~{N}-[[2,4-bis(fluoranyl)phenyl]methyl]-4-[(4-methylpiperazin-1-yl)methyl]aniline 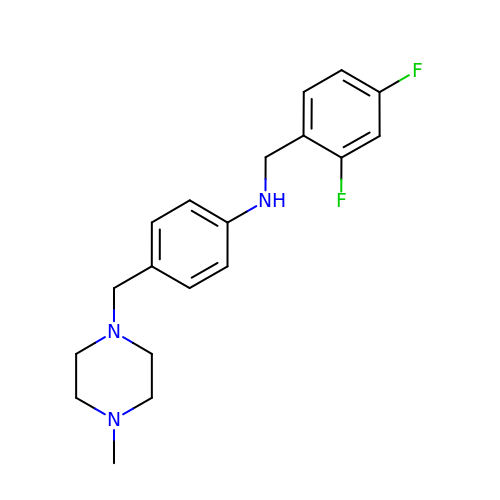| C19 H23 F2 N3 | KZQGQNIDRAAHOA-UHFFFAOYSA-N> PISPIETVPVKLKPGMDGPKVKQWPLTEEKIK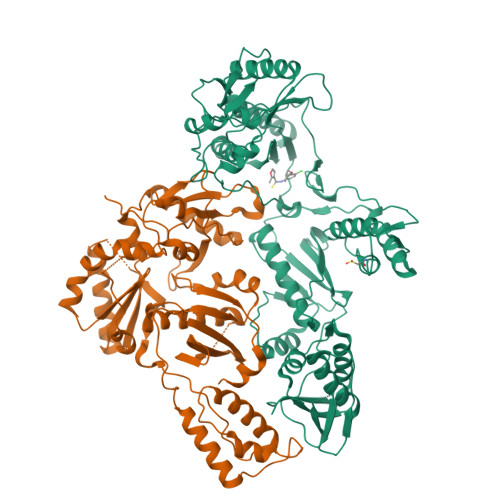ALVEICTEMEKEGKISKIGPENPYNTPVFAIKKKDSTKWRKLVDFRELNKRTQDFWEVQLGIPHPAGLKKKKSATVLDVGDAYFSVPLDEDFRKYTAFTIPSINNETPGIRYQYNVLPQGWKGSPAIFQSSMTKILEPFRKQNPDIVIYQYMDDLYVGSDLEIGQHRTKIEELRQHLLRWGLTTPDKKHQKEPPFLWMGYELHPDKWTVQPIVLPEKDSWTVNDIQKLVGKLNWASQIYPGIKVRQLCKLLRGTKALTEVIPLTEEAELELAENREILKEPVHGVYYDPSKDLIAEIQKQGQGQWTYQIYQEPFKNLKTGKYARMRGAHTNDVKQLTEAVQKITTESIVIWGKTPKFKLPIQKETWETWWTEYWQATWIPEWEFVNTPPLVKLWYQLEKEPIVGAETFYVDGAANRETKLGKAGYVTNRGRQKVVTLTDTTNQKTELQAIYLALQDSGLEVNIVTDSQYALGIIQAQPDQSESELVNQIIEQLIKKEKVYLAWVPAHKGIGGNEQVDKLVSAGIRKVL;> PISPIETVPVKLKPGMDGPKVKQWPLTEEKIKALVEICTEMEKEGKISKIGPENPYNTPVFAIKKKDSTKWRKLVDFRELNKRTQDFWEVQLGIPHPAGLKKKKSATVLDVGDAYFSVPLDEDFRKYTAFTIPSINNETPGIRYQYNVLPQGWKGSPAIFQSSMTKILEPFRKQNPDIVIYQYMDDLYVGSDLEIGQHRTKIEELRQHLLRWGLTTPDKKHQKEPPFLWMGYELHPDKWTVQPIVLPEKDSWTVNDIQKLVGKLNWASQIYPGIKVRQLCKLLRGTKALTEVIPLTEEAELELAENREILKEPVHGVYYDPSKDLIAEIQKQGQGQWTYQIYQEPFKNLKTGKYARMRGAHTNDVKQLTEAVQKITTESIVIWGKTPKFKLPIQKETWETWWTEYWQATWIPEWEFVNTPPLVKLWYQLEKEPIVGAETF> MIMPQHDQLHRYLFENFAVRGELVTVSETLQQILENHDYPQPVKNVLAELLVATSLLTATLKFD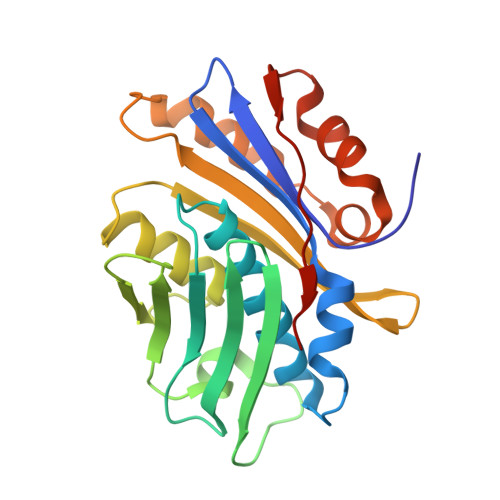GDITVQLQGDGPMNLAVINGNNNQQMRGVARVQGEIPENADLKTLVGNGYVVITITPSEGERYQGVVGLEGDTLAADLEDYFMRSEELPTRLFIRTGDVDGKPAAGGMLLQVMPAQNAQQDDFDHLATLTETIKTEELLTLPANEVLWRLYHEEEVTVYDPQDVEFKCTCS>MVPPTINTGKNITTERAVLTLNGLQIKLHKVVGESRDDIVAKMKDLAMDDHKFPRLPGPNPVSIERKDFEKLKQNKYVVSEKTDGIRFMMFFTRVFGFKVCTIIDRAMTVYLLPFKNIPRVLFQGSIFDGELCVDIVEKKFAFVLFDAVVVSGVTVSQMDLASRFFAMKRSLKEFKNVPEDPAILRYKEWIPLEHPTIIKDHLKKANAIYHTDGLIIMSVDEPVIYGRNFNLFKLKPGTHHTIDFIIMSEDGTIGIFDPNLRKNVPVGKLDGYYNKGSIVECGFADGTWKYIQGRSDKNQANDRLTYEKTLLN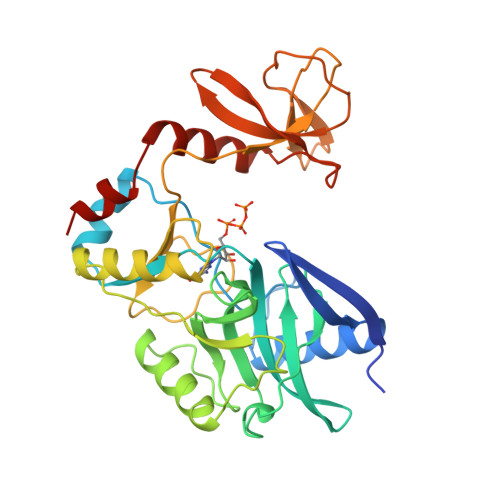IEENITIDELLDLFKWE[2x]> GIPRRITKETQNLANEPPPGIMAVPVPENYRHFNILINGPDGTPYEGGTYKLELFLPEQYPMEPPKVRFLTKIYHPNIDKLGRICLDILKDKWSPALQIRTVLLSIQALLSSPEPDDPLDSKVAEHFK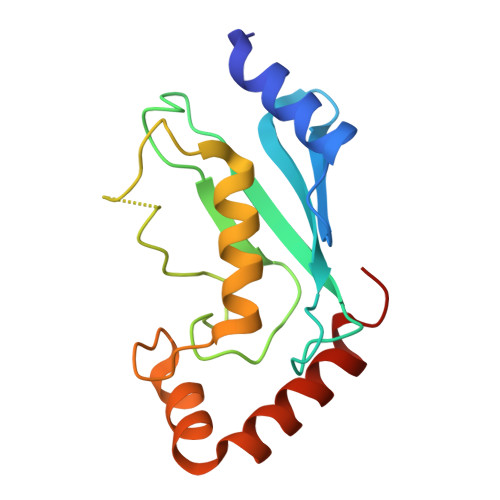QDKNDAEHVARQWNKIYANNNVL>MNTISILSTTDLPAAWQIEQRAHAFPWSEKTFFGNQGERYLNLKLTADDRMAAFAITQVVLDEATLFNIAVDPDFQRRGLGRMLLEHLIDELETRGVVTLWLEVRASNAAAIALYESLGFNEATIRRNYYPTAQGHEDAIIMALPISMKLHH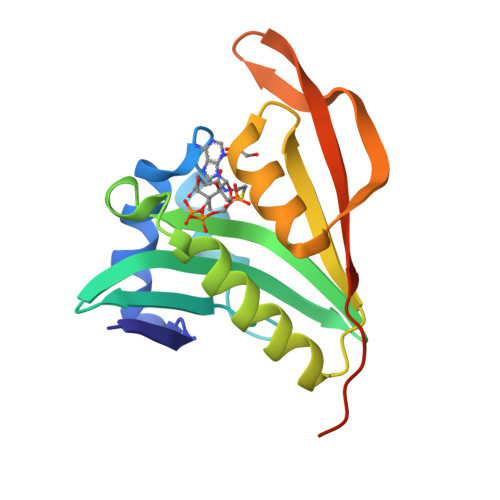HHHHHHHH[4x]> ADTIVAVELDSYPNTDIGDPSYPHIGIDIKSIRSKATARWNMQTGKVGTAHISYNSVAKRLSAVVSYSGTSSTTVSYDVDLNNVLPEWVRVGLSATTGLYKETNTILSWSFTSKLKTNSIADANSLHFSFNQFSQNPKDLILQGDATTDSDGNLQLTRVSSDGSPQGSSVGRALFYAPVHIWEKSAVVASFDATFTFLIK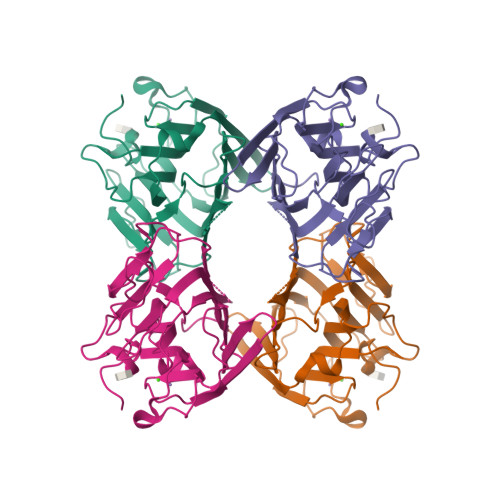SPDRDPADGITFFIANTDTSIPSGSGGRLLGLFPDAN>[2x]MVSVSEIRKAQRAEGPATILAIGTANPANCVEQSTYPDFYFKITNSEHKTELKEKFQRMCDKSMIKRRYMYLTEEILKENPNVCEYMAPSLDARQDMVVVEVPRLGKEAAVKAIKEWGQPKSKITHLIVCTTSGVD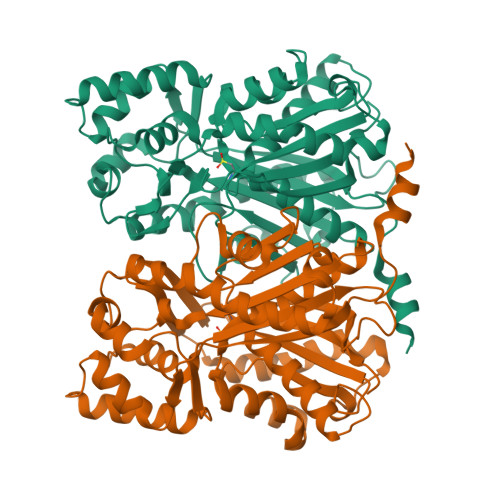MPGADYQLTKLLGLRPYVKRYMMYQQGCFAGGTVLRLAKDLAENNKGARVLVVCSEVTAVTFRGPSDTHLDSLVGQALFGDGAAALIVGSDPVPEIEKPIFEMVWTAQTIAPDSEGAIDLHLREAGLTFHLLKDVPGIVSKNITKALVEAFEPLGISDYNSIFWIAHPGGPAILDQVEQKLALKPEKMNATREVLSEYGNMSSACVLFILDEMRKKSTQNGLKTTGEGLEWGVLFGFGPGLTIETVVLRSVAI>GPLPVDLRGKTAFVAGVADSNGYGWAICKLLRAAGARVLVGTWPPVYSIFKKGLESSRFEQDSFYAQEPSSKVAAEAAEKPVDLVFDKIYPLDAVFDTPQDVPPEVSSNKRYAGVGGFTISEVAEAVRADVGQIDILVHSLANGPEVTKPLLQTSRKGYLAAVSSSSYSFVSLLQHFLPLMKEGGSALALSYIASEKVIPGYGGGMSSAKAALESDCRTLAFEAGRAR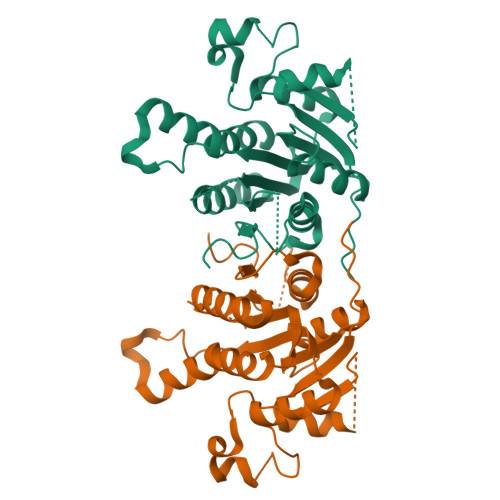AVRVNCISAGPLKSRAASAIGKAGDKTFIDLAIDYSEANAPLQKELESDDVGRAALFLLSPLARAVTGATLYVDNGLHAMGQALDSKSLTP[2x]> GSHMEFDERDRVQKKTFTKWVNKHLIKHWRAEAQRHISDLYEDLRDGHNLISLLEVLSGDSLPREKGRMRFHKLQNVQIALDYLRHRQVKLVNIRNDDIADGN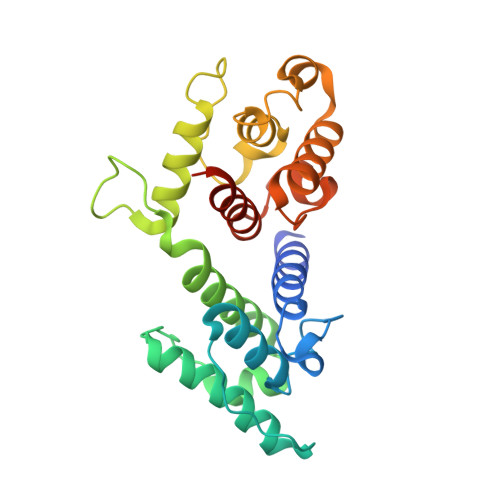PKLTLGLIWTIILHFQISDIQVSGQSEDMTAKEKLLLWSQRMVEGYQGLRCDNFTTSWRDGRLFNAIIHRHKPMLIDMNKVYRQTNLENLDQAFSVAERDLGVTRLLDPEDVDVPQPDEKSIITYVSSLYDAMPRVPGAQEF>MGSSHHHHHHSSGDHRKIGRDQELYFFHELSPGSCFFLPKGAYIYNALIEFIRSEYRKRGFQEVVTPNIFNSRLWMTSGHWQHYSENMFSFEVEKELFALKPMNCPGHCLMFDHRPRSWRELPLRLADFGVLHRNELSGALTGLTRVRRFQQDDAHIFCAMEQIEDEIKGCLDFLRTVYSVFGFSFKLNLSTRPEKFLGDIEVWDQA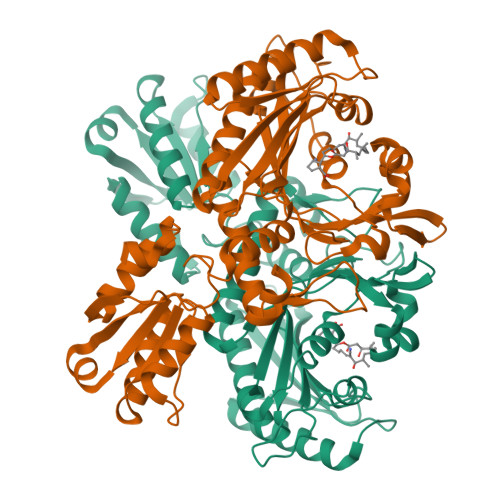EKQLENSLNEFGEKWELNSGDGAFYGPKIDIQIKDAIGRYHQCATIQLDFQLPIRFNLTYVSHDGDDKKRPVIVHRAILGSVERMIAILTENYGGKWPFWLSPRQVMVVPVGPTCDEYAQKVRQQFHDAKFMADIDLDPGCTLNKKIRNAQLAQYNFILVVGEKEKISGTVNIRTRDNKVHGERTISETIERLQQLKEFRSKQAEEEF[4x]> MTDLRKLEALQALHAELVAVRQHRFEGLQVLETLLEEQTDAFKALIAKPARDTKDREALGKEPKKLKIGEEEYSLNEDFVNDCLKLADELDLNEKESARILIDCDAEGDVETQSRPLWECGVIRFHQERKYLLDCMRLILEIAADEDIDAGLQESFGVAAEDKIFGIPPPWERNKENQPTQVKKFIPRCMEAMKGVRSMLQCMADKANARNMLQQASLVRPLDNQETLDFSRLSLVEQHECLASILHAAVQRHHATIADFQDFIKILRKWDKYDHFLIHLIPVLAAYITEFGSPEGMGDLQQARRLNDFICKGGDEDSWALPVLGAAVRAWWIAEHNGFYLDDTVQDLRGINLDEEDEQRTKQFLDALKEGAFDFILSVAADCKAQEWQDPSQLG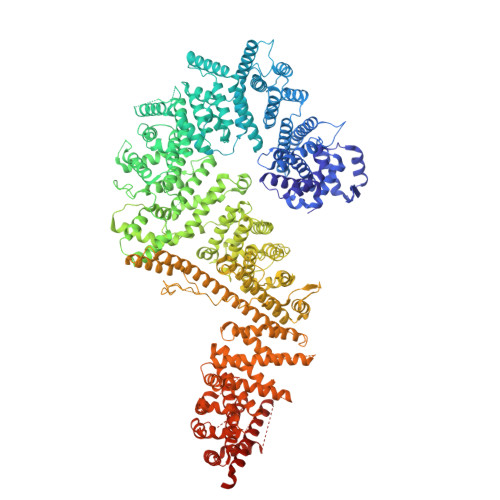ARQWLQRKIPSLPSEPFPFSHFLQHSLMVHLEGFVDATISNLPDVLRKLRTEEDEQRQLRPNHEQDMDLERFLIIISYAYEGRPDAAMSFWEDPDSNLAGFLQWASRRASTPLVSAFCEMLRCLADNEECATAAHNFLLDEGHQASGKMKRSQSLTWSQIFKELEYFTTKVCSERPNPPQASMHRPGRPGADPAEIEPESALMLECYLRLIAKLATESEIARKRLIMDEDFNLVDTILKLSVGVIPHRLRACIFYVLKALMIRKTHEELDAMWRWVEAWMTNPFSSLPGSQGAPQRISFLGQTPGPQECMEMMFREFGTGFEQSNAFIQLLTTLLVPPEGLNSLNDSVPFPEWLGSSIRTLGIEPYVDFVFDVFANRTKDISDPSQLRILRLSCLDFVMVCLVTFNEDLIVLGHESNISIDDAMAATNLATYVRLHPFSRVMEWLFNEKVITSLINTIHQDPISLGSASPDSPLVVSILRAIQVMIKALELQETYLHLVRPEVLRYQGEAGVRRKPVANAAYSAFEDGILSHLSLVVDLGKYCNLGHAELTLACLKLLEKISTSSRILSAWSPDSGRLGHRNKAIVQLERNGEGETISASLSASIMATLDPALAASGENYRVKLAILDFLYACLRATPDQPTIAHQLLGFHCELSKLGIEPKGPFDMQKSLFHSLLNVLITLTVSEEEQGMRGYLVTLKYRVLRILQLLWKSPLSASLVMDELRATNFLFHMLLREVQIQPQLPWDGQLVTGCEFLLSDASLAYIDYLASRAAIFEYIGKELCSVSQNRIPSIKRQIFDALNGQIFVDEEAPLTIPSIFDFFDFINTDYKWEEIPSPHFTYLKDLDLGPCILEHKYAGVHYDIRKAQEILALKRKEYEHSQLATPEFLETVELEEKVLIEWLTVRNRANLLLTARLNLLQAWANLLLVMIESNDFKSTPKMAFLLQALQAILPTLEAFSSLKSDEAFELARVAKVLLWKLDFSQDSDAGLDREQFTVGNLIGDKLFQLFQLCLSAISQCSGTPELRSLYYSICYRYLTAVVDNDATVAATPASSTIGPTRSVTNARARTLKAITLYGDRLLNVICDDAYGSDTTCQTAAMILLNALVHTSRASSAAGVSPADVDCPIIDALNRLNFIGVLVDSLKEILNEWLAPSSTFDPSLSTNASPSLPIPASPSQQYTSAKLALLLQLCQTRQGAKYVLQANLFRALEQSGVFAADPELVEVDSESGVPRVVALERHYALLVALARVVGAAVTARGAHNIVQGRKFLTQHRGLVVHVLKKNAGIGGGVVGNSLASSINGGSTATMTRRDEILAQQALEERIEELAEAFMLLITATGFLEYESEQVPSEQPRAHTTFFH> GAMGSGIPMEACPHIRYAFQNDKLLLQQASVGRLTLVNKTTILLRP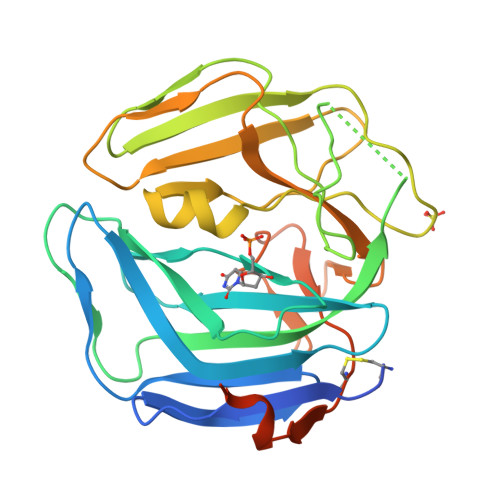MKTTTVDLGLYARPPEGHGLMLWGSTSRPVTSHVGIIDPDYTGELRLILQNQRRYNSTLRPSELKIHLAAFRYATPQMEEDKGPINHPQYPGSVGLDVSLPKDLALFPHQTVSVTLTVPPPSIPHHRPTIFGRSGLAMQGILVKPCRWRRGGVDVSLTNFSDQTVFLNKYRRFCQLVYLHKHHLTSFYSPHSDAGVLGPRSLFRWASCTFEEVPSLAMGDSGLSEALEGRQGRGFGSSGQ> Q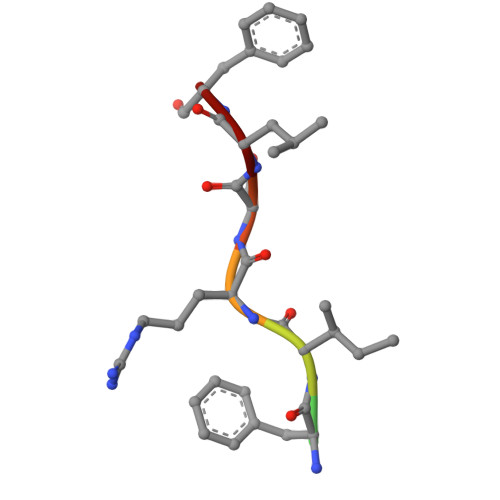EFIRSLF3-[4-[(2~{R},3~{S},4~{S},5~{S},6~{R})-6-(hydroxymethyl)-3,4,5-tris(oxidanyl)oxan-2-yl]oxy-3-methyl-phenyl]-~{N}-methyl-benzamide 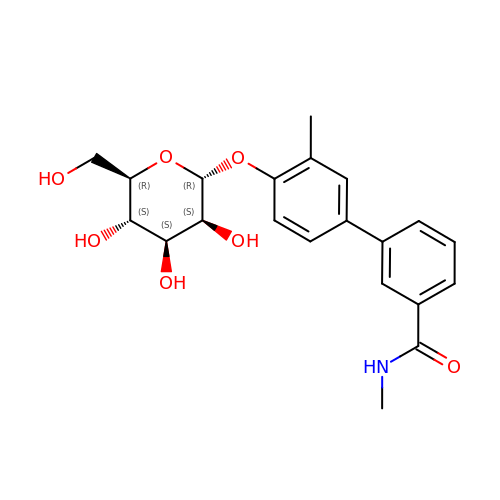| C21 H25 N O7 | LECOXVSYFKTZFV-AGRFSFNASA-N> HMSPSPVPGSQNVPAPAVKKISQYACQRRTTLNNYNQLFTDALDILAENDELRENEGSCLAFMRASSVLKSLPFPITSMKDTEGIPCLGDKVKSIIEGIIEDGESSEAKAVLNDERYKS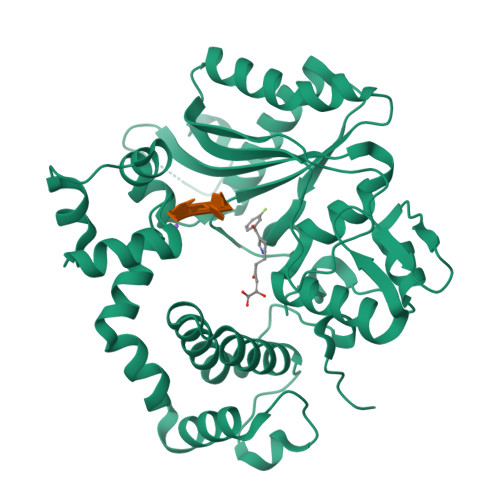FKLFTSVFGVGLKTAEKWFRMGFRTLSKIQSDKSLRFTQMQKAGFLYYEDLVSCVNRPEAEAVSMLVKEAVVTFLPDALVTMTGGFRRGKMTGHDVDFLITSPEATEDEEQQLLHKVTDFWKQQGLLLYCDILESTFEKFKQPSRKVDAADHFQKCFLILKLDHGRVHSEKSGQQEGKGWKAIRVDLVMCPYDRRAFALLGWTGSRQFERDLRRYATHERKMMLDNHALYDRTKRVFLEAESEEEIFAHLGLDYIEPWERNAMGSSHHHHHHSSGLVPRGS>[2x]GMSGGGEQLDILSVGILVKERWKVLRKIGGGG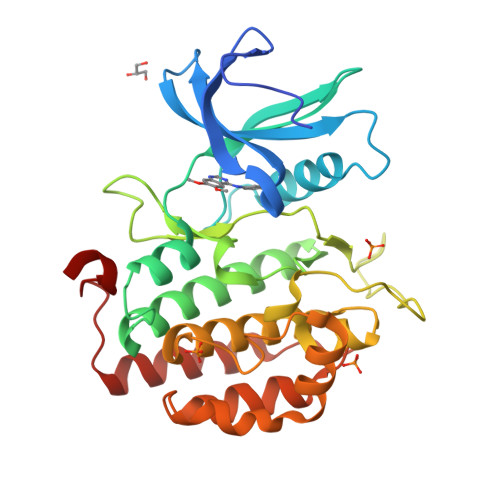FGEIYDALDMLTRENVALKVESAQQPKQVLKMEVAVLKKLQGKDHVCRFIGCGRNDRFNYVVMQLQGRNLADLRRSQSRGTFTISTTLRLGRQILESIESIHSVGFLHRDIKPSNFAMGRFPSTCRKCYMLDFGLARQFTNSCGDVRPPRAVAGFRGTVRYASINAHRNREMGRHDDLWSLFYMLVEFVVGQLPWRKIKDKEQVGSIKERYDHRLMLKHLPPEFSIFLDHISSLDYFTKPDYQLLTSVFDNSIKTFGVIESDPFDWEK>[3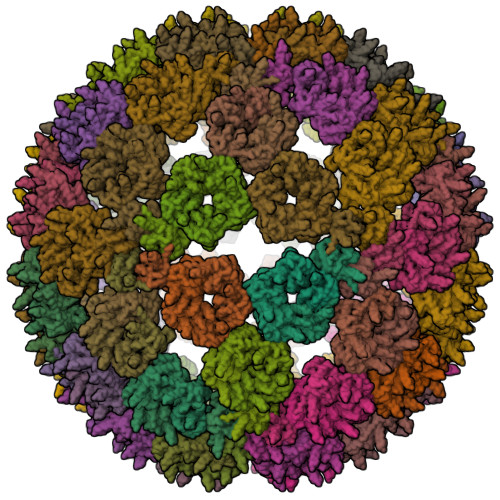60x]MEIYEGKLTAEGLRFGIVASRFNHALVGRLVEGAIDCIVRHGGREEDITLVCVPGSWEIPVAAGELARKEDIDAVIAIGVLIEGAEPHFDYIASEVSKGLANLSLELRKPISFGDITDDELEEAIECAGTEHGNKGWEAALSAIEMANLFKSLRLEHHHHH5-[1-(1,3-dimethoxypropan-2-yl)-5-morpholin-4-yl-benzimidazol-2-yl]-1,3-dimethyl-pyridin-2-one 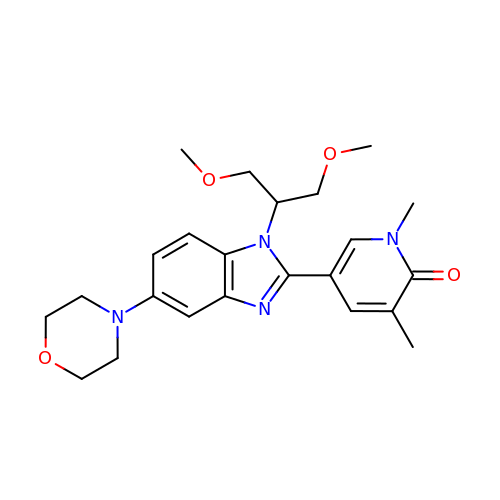| C23 H30 N4 O4 | DDSHVVXWYKDTTQ-UHFFFAOYSA-N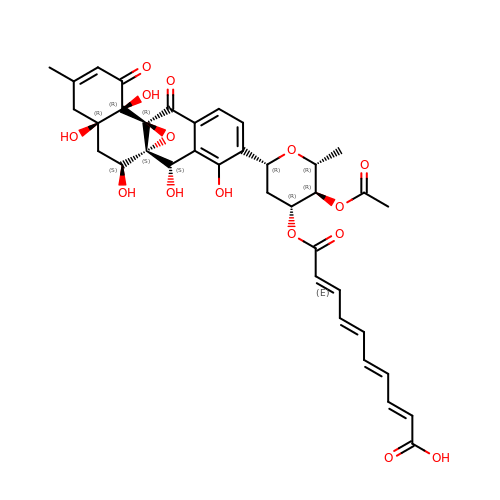SIMOCYCLINONE C4 | C37 H38 O15 | FTHVOUWMLYLIFE-WSOZGFGQSA-N> MQDITM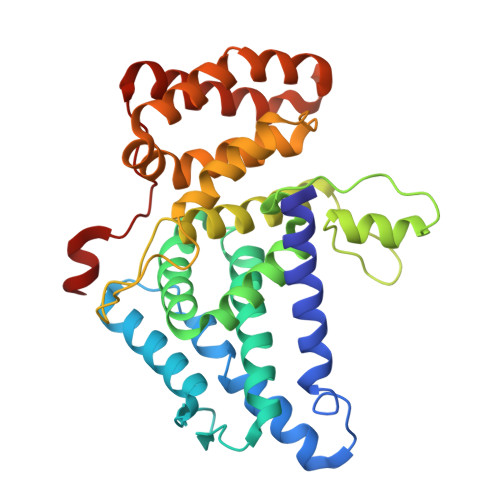QWYQQLQDASMQCVLTFEGLTNSKDSQAKKIKMDLQKAATIPVSQISTIAGSKLKEIFDKIHSLLSGKPVQSGGRSVSVTLNPQGLDFVQYKLAEKFVKQGEEEVASHHEAAFPIAVVASGIWELHPRVGDLILAHLHKKCPYSVPFYPTFKEGMALEDYQRMLGYQVKDSKVEQQDNFLKRMSGMIRLYAAIIQLRWPYGNRQEIHPHGLNHGWRWLAQILNMEPLSDVTATLLFDFLEVCGNALMKQYQVQFWKMLILIKEDYFPRIEAITSSGQMGSFIRLKQFLEKCLQHKDIPVPKGFLTSSFWRS> MAKINELLRESTTTNSNSIGRPNLVALTRATTKLIYSDIVATQRTNQPVAAFYGIKYLNPDNEFTFKTGATYAGEAGYVDREQITELTEESKLTLNKGDLFKYNNIVYKVLEDTPFATIEESDLELALQIAIVLLKVRLFSDAASTSKFESSDSEIADARFQINKWQTAVKSRKLKTGITVELAQDLEANGFDAPNFLEDLLATEMADEINKDILQSLITVSKRYKVTGITDSGFIDLSY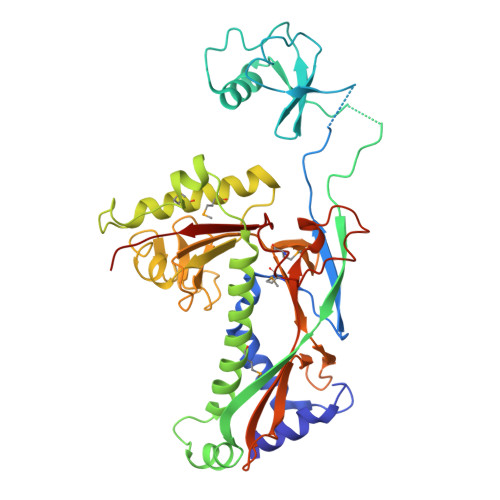ASAPEAGRSLYRMVCEMVSHIQKESTYTATFCVASARAAAILAASGWLKHKPEDDKYLSQNAYGFLANGLPLYCDTNSPLDYVIVGVVENIGEKEIVGSIFYAPYTEGLDLDDPEHVGAFKVVVDPESLQPSIGLLVRYALSANPYTVAKDEKEARIIDGGDMDKMAGRSDLSVLLGVKLPKIIIDE5-fluoropyrimidin-2-ol | C4 H3 F N2 O | 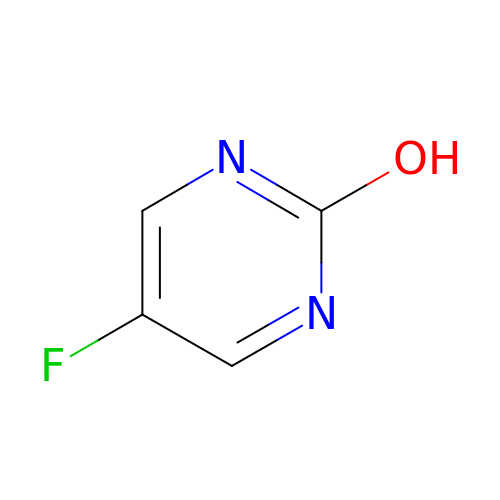HPABFFGQPLJKBP-UHFFFAOYSA-N>MTQTAAKSLKFPKDFLWGAATAAYQIEGAANEDGRGPSIWDTFSHTPGKVHNGDNGDVACDHYHRYKEDVELMKELGLNAYRFSISWPRILPEGEGKVNQKGLDFYNNLIDELLENGIEPFVTLYHWDLPQALQDKGGWENRETVDAFAEYARVCFERFGDRVKYWITFNEPNVFAVLGYLSGVHPPGMKDLKKAFRAAHNLLLAHARAVKAYREISQNGQIGITLNLSPVYPASDNEEEDKAAAERADQFNNWFLDPIFKGKYEHMLERLGEQIAANGGELPEITDEMEILSASLDFIGLNYYTSNLVRANPNSG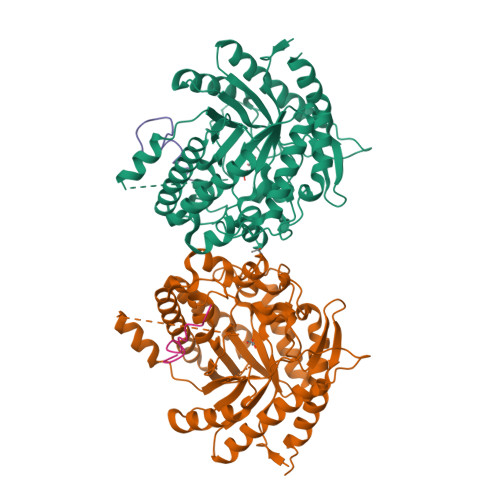SSSVKPPDLPRTDMGWEIYPEGLYDLLKRIHEKYNLPIYITENGMAVDDEVEDGAVHDTNRIDYLKEHLEAVHKAIEEGVNVRGYFVWSLMDNFEWANGYSKRFGLIYVDYKTQKRTPKKSAYWYREVIKSNGLELEHHHHHH[2x]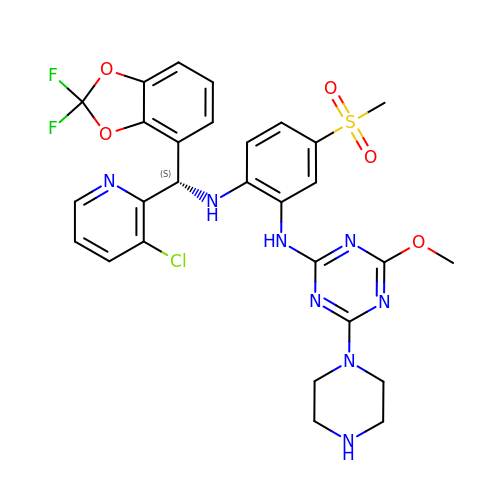~{N}1-[(~{S})-[2,2-bis(fluoranyl)-1,3-benzodioxol-4-yl]-(3-chloranylpyridin-2-yl)methyl]-~{N}2-(4-methoxy-6-piperazin-1-yl-1,3,5-triazin-2-yl)-4-methylsulfonyl-benzene-1,2-diamine | C28 H27 Cl F2 N8 O5 S | QJIMSJUUARCROQ-QFIPXVFZSA-N>[7x]AKDVKFGADARALMLQGVDLLADAVAVTM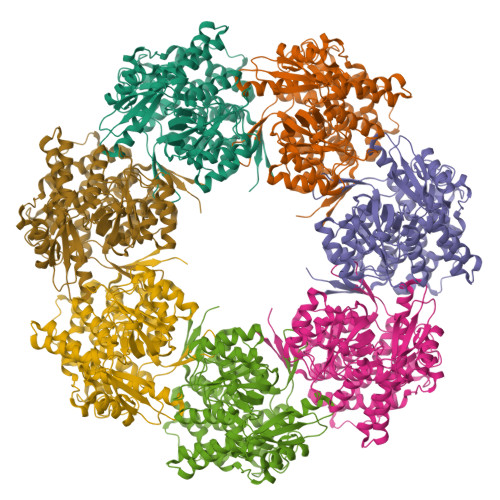GPKGRTVIIEQSWGSPKVTKDGVTVAKSIDLKDKYKNIGAKLIQDVANNTNEEAGDGTTTATVLARSIAKEGFEKISKGANPVEIRRGVMLAVDAVIAELKKQSKPVTTPEEIAQVATISANGDKEIGNIISDAMKKVGRKGVITVKDGKTLNDELEIIEGMKFDRGYISPYFINTSKGQKCEFQDAYVLLSEKKISSIQSIVPALEIANAHRKPLVIIAEDVDGEALSTLVLNRLKVGLQVVAVKAPGFGDNRKNQLKDMAIATGGAVFGEEGLTLNLEDVQPHDLGKVGEVIVTKDDAMLLKGKGDKAQIEKRIQEIIEQLDVTTSEYEKEKLNERLAKLSDGVAVLKVGGTSDVEVNEKKDRVTDALNATRAAVEEGIVLGGGCALLRCIPALDSLTPANEDQKIGIEIIKRTLKIPAMTIAKNAGVEGSLIVEKIMQSSSEVGYDAMAGDFVNMVEKGIIDPTKVVRTALLDAAGVASLLTTAEVVVTEIP> GQKIGILGAMREEITPILELFGVDFEEIPLGGNVFHKGVYHNKEIIVAYSKIGKVHSTLTTTSMILAFGVQKVLFSGVAGSLVKDLKINDLLVATQLVQHDVDLSAFDHPLGFIPESAIFIETSGSLNALAKKIANEQHIALKEGVIASGDQFVHSKERKEFLVSEFKASAVEMEGASVAFVCQKFG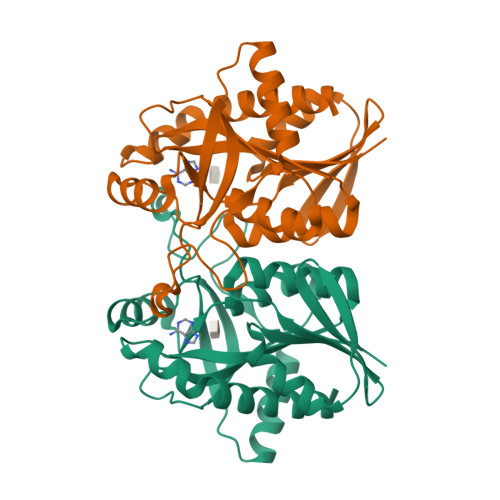VPCCVLRSISDNADEKAGMSFDEFLEKSAHTSAKFLKSMVDEL> CTDAALAALEYHK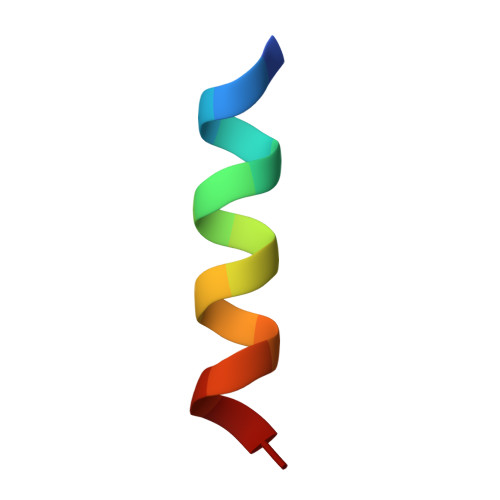SNA N-{3-[(4S,6S)-2-amino-4-methyl-6-(trifluoromethyl)-5,6-dihydro-4H-1,3-oxazin-4-yl]-4-fluorophenyl}-5-cyanopyridine-2-carboxamide 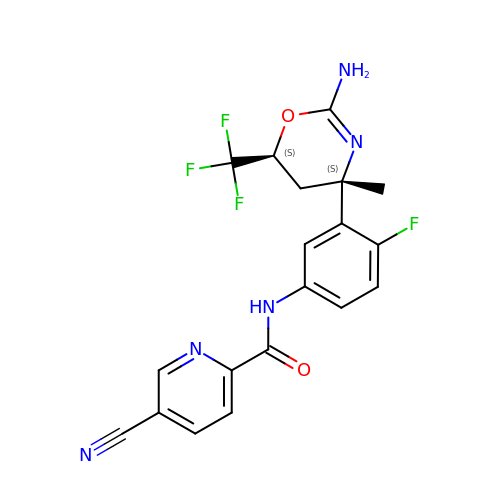| C19 H15 F4 N5 O2 | MELQHVBGGSKVJQ-YJBOKZPZSA-N> MVPMDKTLKEFGADVQWDDYAQLFTLIKDGAYVKVKPGAQTAIVNGQPLALQVPVVMKDNKAWVSDTFINDVFQSGLDQTFQVEKRPHPLNALTADEIKQAVEIV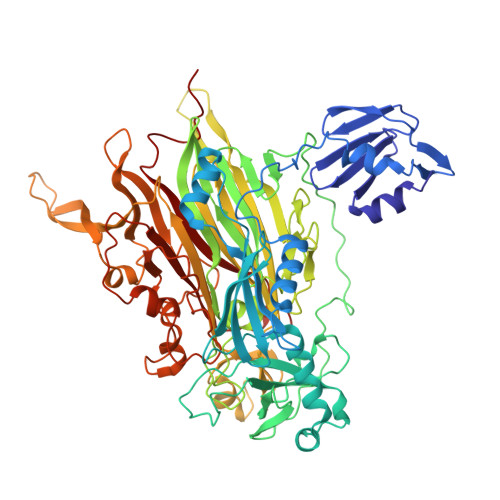KASADFKPNTRFTEISLLPPDKEAVWAFALENKPVDQPRKADVIMLDGKHIIEAVVDLQNNKLLSWQPIKDAHGMVLLDDFASVQNIINNSEEFAAAVKKRGITDAKKVITTPLTVGYFDGKDGLKQDARLLKVISYLDVGDGNYWAHPIENLVAVVDLEQKKIVKIEEGPVVPVPMTARPFDGRDRVAPAVKPMQIIEPEGKNYTITGDMIHWRNWDFHLSMNSRVGPMFSTVTYNDNGTKRKVMYEGSLGGMIVPYGDPDIGWYFKAYLDSGDYGMGTLTSPIARGKDAPSNAVLLNETIADYTGVPMEIPRAIAVFERYAGPEYKHQEMGQPNVSTERRELVVRWISTVGNYDYIFDWIFHENGTIGIDAGATGIEAVKGVKAKTMHDETAKDDTRYGTLIDHNIVGTTHQHIYNFRLDLDVDGENNSLVAMDPVVKPNTAGGPRTSTMQVNQYNIGNQQDAAQKFDPGTIRLLSNPNKENRMGNPVSYQIIPYAGGTHPVAKGAQFAPDEWIYHRLSFMDKQLWVTRYHPGERFPEGKYPNRSTHDTGLGQYSKDNESLDNTDAVVWMTTGTTHVARAEEWPIMPTEWVHTLLKPWNFFDETPTLGALK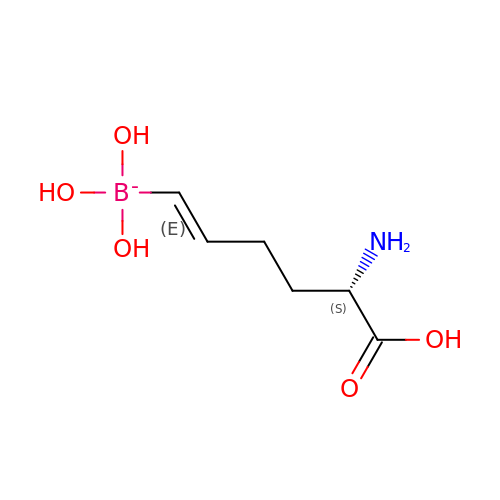[(1E,5S)-5-AMINO-5-CARBOXYPENT-1-ENYL](TRIHYDROXY)BORATE(1-) | C6 H13 B N O5 | CCCYGXMAMSUXAV-FYTLMZHYSA-N>MSDQCVTVEAPINIAFIKYWGKREGGETLILPTNDSFSITLSASPFRSKTSVELRDDIETDTLRLNGTEVDVGKTPRVQS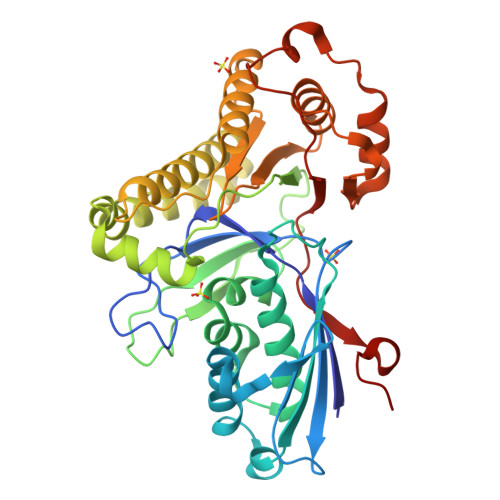MLLHLRSTCPEELKNKKVNIVSENNFPTAAGMASSASGYCAMSAALIRAFKSTTNVSMLARLGSGSACRSAFGGFVIWNKGEKPDGSDCVATQFVDETHWPEIQVMCAVLKGAQKDVSSTKGMQQSLKTSPLMKKRISETVPERMKIASRAIKARDFATFAEIAMLESDDLQEICATTEPKITYATEDSYAMIRLVKAYNAKKGRTALAYTFDAGANCFLFVLKEDLPEAVAMLMEHFPTPFEKFFFGDRELLEKVKVVSLPDEYKKLIDHPKKPFEMLLQSPVGCGVKYLGPSESLIPP[2x]> MSDGAVQPDGGQPAVRNERATGSGNGSGGGGGGGSGGVGISTGTFNNQTEFKFLENGWVEITANSSRLVHLNMPESENYRRVVVNNMDKTAVNGNMALDDIHAQIVTPWSLVDANAWGVWFNPGDWQLIVNTMSELHLVSFEQEIFNVVLKTVSESATQPPTKVYNNDLTASLMVALDSNNTMPFTPAAMRSETLGFYPWKPTIPTPWRYYFQWDRTLIPSHTGTSGTPTNIYHGTDPDDVQFYTIENSVPVHLLRTGDEFATGTFFFDCKPCRLTHTWQTNRALGLPPFLNSLPQSEGATNFGDIGVQQDKRRGVTQMGNTNYITEATIMRPAEVGYSAPYYSFEASTQGPFKTPIAAGRGGAQTDENQAADGNPRYAFGRQHGQKTTTTGETPERFTYIAHQDTGRYPEGDWIQNINFNLPVTNDNVLLPTDPIGGKTGINYTNIFNTYGPLTALNNVPPVYPNGQIWDKEFDTDLKPRLHVNAPFVCQNNCPGQLFVKVAPNLTNEYDPDASANMSRIVTYSDFWWKGKLVFKAKLRAS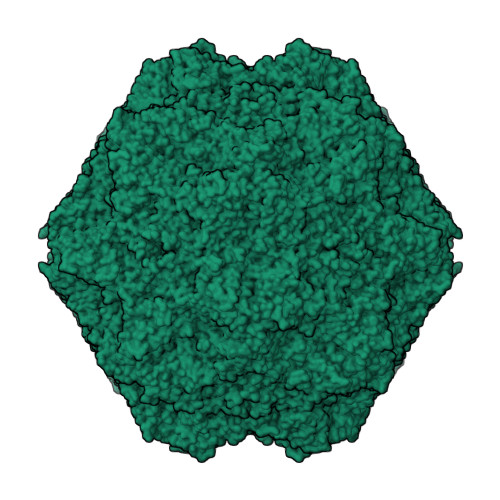HTWNPIQQMSINVDNQFNYVPSNIGGMKIVYEKSQLAPRKLY>[5x]TGGRNSIRYSELAPLFDTTRVYLVDNKSTDVASLNYQNDHSNFLTTVIQNNDYSPGEASTQTINLDDRSHWGGDLKTILHTNMPNVNEFMFTNKFKARVMVSRSLTKDKQVELKYEWVEFTLPEGNYSETMTIDLMNNAIVEHYLKVGRQNGVLESDIGVKFDTRNFRLGFDPVTGLVMPGVYTNEAFHPDIILLPGCGVDFTHSRLSNLLGIRKRQPFQEGFRITYDDLEGGNIPALLDV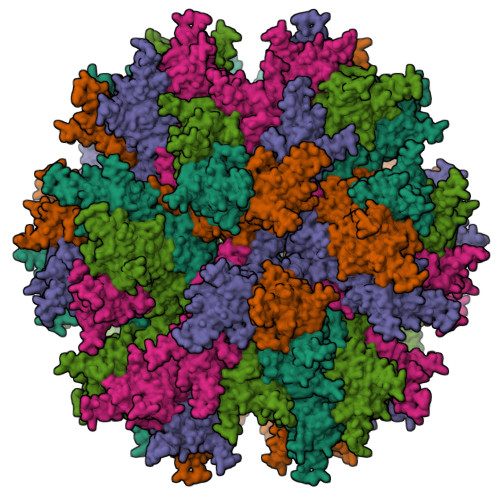DAYQASLKDDTEQGGDGAGGGNNSGSGAEENSNAAAAAMQPVEDMNDHAIRGDTFATRAEEKRAEAEAAAEAAAPAAQPEVEKPQKKPVIKPLTEDSKKRSYNLISNDSTFTQYRSWYLAYNYGDPQTGIRSWTLLCTPDVTCGSEQVYWSLPDMMQDPVTFRSTSQISNFPVVGAELLPVHSKSFYNDQAVYSQLIRQFTSLTHVFNRFPENQILARPPAPTITTVSENVPALTDHGTLPLRNSIGGVQRVTITDARRRTCPYVYKALGIVSPRVLSSRTF> SALV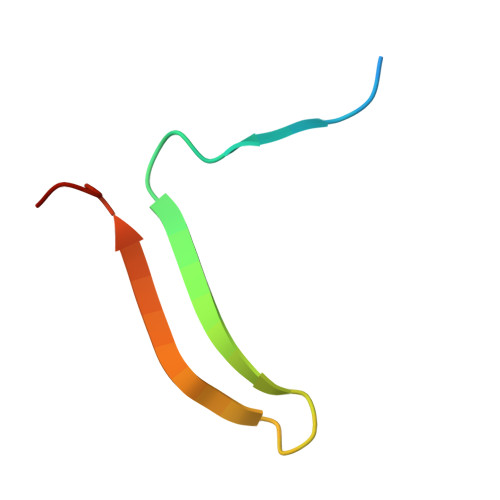ETRTIVRFNRPFLMIIVDHFTWSIFFMSKVTNPKQA> ETGDVKPDLQTKQDKVLAHFIGNSTDYFKILDHNDEFVLVGAKDVIYNVSLNGLKEIARLEWHSTDADRELCALKGKHEWDCHNYLRVYALRPNGEVLLCGTNSYKPRCRHYTPVEVSSEEAGSAGHAHAMRYEVSRDVEAQGLCPYSPAHNSTYAFADGHLYSATVADFSGGDPLIYRENLRTEQYDLKQLNQPDFVGAIERNGYVLFFFRELSMEVMNFGKAVYSRVARVCKNDRGGPYSHGKSWTSFLKARLNCSVPGEFPFYFDEIQAISPIVESGSKSLIYAVFTTSVNAIPGSAVCAFNVDDILAAFDGEFKSQKDSQSHWLPVEREQVPKPRPGQCVEDSRTLTSIAVNFIKNHPLMEEAVPAVHGRPLLTKVNLHHRLTAIAVHPQVKSLSGAYYDVIYSGTDDGKVTKFINILSTHPNSTVDRLKTVVISEMQVLPLGTPIRELVISTSKNSLVVVSDGSLVSVPLHHCSHIVDCLGCLSLQDPICAWDLQTHECKNLATSQHKFGTKTYLQSLNSTKKAAALLCPHIPR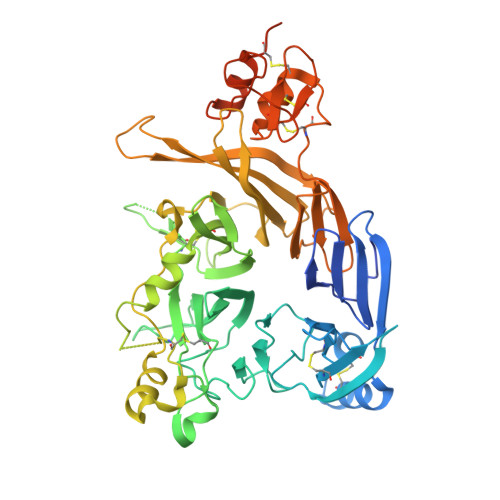DAPGAETVSFVTMAPPPTEEQKLLYSNVGSGTKHHHHHH> MNHEPEVKATDMEEDMIKRVK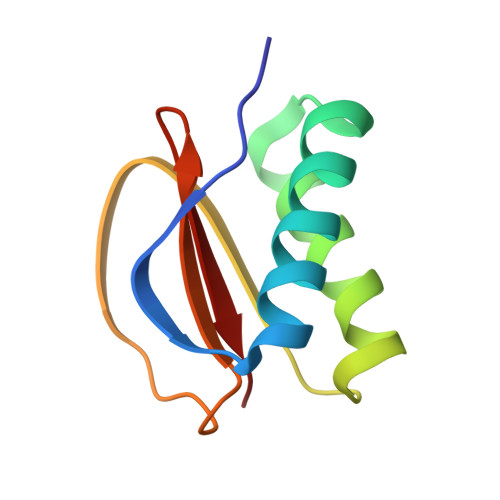EIAINAVKEYKQEKQIAHYIKYEFDKIDGYGWNCIVGRNFGSHIIHQTKKYIFFKINELCLLLWKA>[3x]PAAAA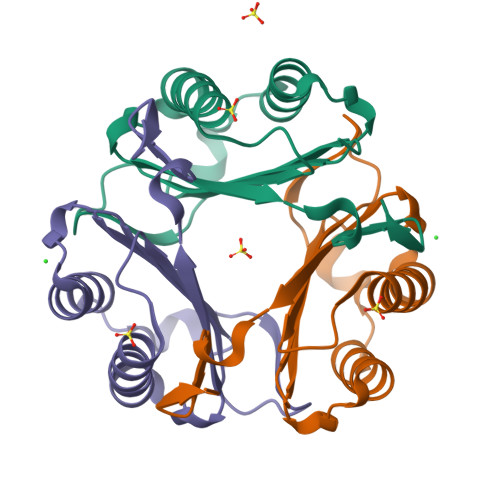MFIVNTNVPRASVPDGFLSELTQQLAQATGKPPQYIAVHVVPDQLMAFGGSSEPCALCSLHSIGKIGGAQNRSYSKLLCGLLAERLRISPDRVYINYYDMNAANVGWNNSTFA4-[(4-amino-5-cyano-6-ethoxypyridin-2-yl)amino]benzamide 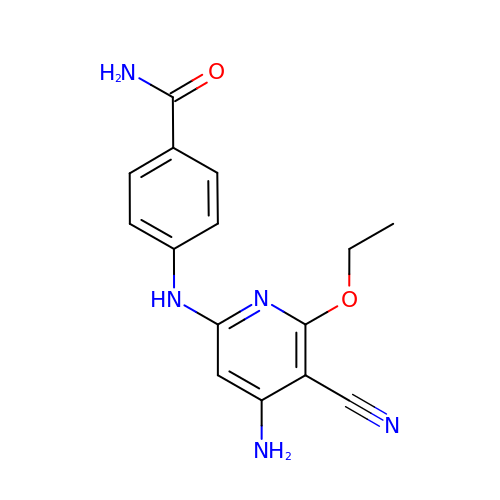| C15 H15 N5 O2 | JUNWGTQNFTURHK-UHFFFAOYSA-N>[7x]GSAKDVKFGADARALMLQGVDLLADAVAVTMGPKGRTVIIEQSWGSPKVTKDGVTVAKSIDLKDKYKNIGAKLVQDVANNTNEEAGDGTTTATVLARSIAKEGFEKISKGANPVEIRRGVMLAVDAVIAELKKQSKPVTTPEEIAQVATISANGDKEIGNIISDAMKKVGRKGVITVKDGKTLNDELEIIEGMKFDRGYISPYFINTSKGQKCEFQDAYVLLSEKKISSIQSIVPALEIANAHRKPLVIIAEDVDGEALSTLVLNRLKVGLQVVAVKAPGFGDNRKNQLKDMAIATGGAVFGEEGLTLNLEDVQPHDLGKVGEVIVTKDDAMLLKGKGDKAQIEKRIQEIIEQLDVTTSEYEKEKLNERLAKLSDGVAVLKVGGTSDVEVNEKKDRVTDALNATRAAVEEGIVLGGGCALLRCIPALDSLTPANEDQKIGIEIIKRTLKIPAMTIAKNAGVEGSLIVEKIMQSSSEVGYDAMAGDFVNMVEKGIIDPTKVVRTALLDAAGVASLLTTAEVVVTEIPKE;>GQAFRKFLPLFDRVLVERSAAETVTKGGIMLPEKSQGKVLQATVVAVGSGSKGKGGEIQPVSVKVGDKVLLPEYGGTKVVLDDKDYFLFRDGDILGKYVD[7x]

The group I mitochondrial chaperonin mHsp60 and its co-chaperonin mHsp10 assist the folding of mitochondrial-imported proteins, and correct misfolded polypeptides resulting from mitochondrial stress. Like GroEL, human mHsp60 can also assemble into stacked back-to-back double-heptameric rings capped by a dome-shaped heptameric mHsp10 (GroES in the case of E. coli) co-chaperonin lid to form ATP-driven nanocages for a substrate–protein to fold in confinement. Features shared by all three structures include mHsp60 protomers in an extended conformation along the molecular symmetry axis with clearly defined domains, namely an equatorial ATP-binding domain (residues 1–137, 411–526), an intermediate hinge domain (residues 138–191, 375–411), and an apical domain (residues 192–374). Each mHsp10 protomer adopts the canonical seven-strand β-barrel structure and exposes a flexible loop sequence of twenty residues (mobile loop) that mediates the interaction with helices H and I of the mHsp60 apical domains.

Two-dimensional (2D) classification revealed that mHsp60 and mHsp10 assembled primarily into football complexes accounting for ~70% of the particles, followed by half-football complexes (~30% of the particles). Independently of the football complexes, we also determined a 3.83 Å resolution C7 symmetry 3D reconstruction of the half-football complexes observed in this data set (EMD-9196). The specific amino acid interactions with ADP and Mg2+ mirror those reported in the ADP-bound crystal mHsp60E321K–mHsp10 structure, except that in our map several water molecules are also visible. The same ADP-bound nucleotide state is found in the half-football (stage V). The differences between the ADP football and half-football are quite small (RMSD ~0.5 Å), and indicate that these structures are essentially the same, saving for the quaternary structure difference (football vs. half-football). However, all the nucleotide-binding sites in our football and half-football WT mHsp60–mHsp10 structures were occupied by ADP, indicating that under our specimen preparation conditions ATP hydrolysis had occurred rapidly. The structures of the ADP footballs and half-footballs provide potential evidence for a second level of structural dynamics along the reaction cycle, namely the inter-ring split of mHsp60–mHsp10 football complexes. Our SEC-MALS analysis and the cryo-EM structures of the ADP football and half-football complexes are consistent with these findings. We also provided structural details of half-football complexes, and experimental evidence suggesting that active single- and double-ring mHsp60 complexes coexist in the reaction cycle of the human mHsp60–mHsp10 chaperonin system.>[2x]MGATGDAEQPRGPSGAERGGLELGDAGAAGQLVLTNPWNIMIKHRQVQRRGRRSQMTTSFTDPAISMDLLRAVLQPSINEEIQTVFNKYMKFFQKAALNVRDNVGEEVDAEQLIQEACRSCLEQAKLLFS;>[2x]MAQTQGTRRKVCYYYDGDVG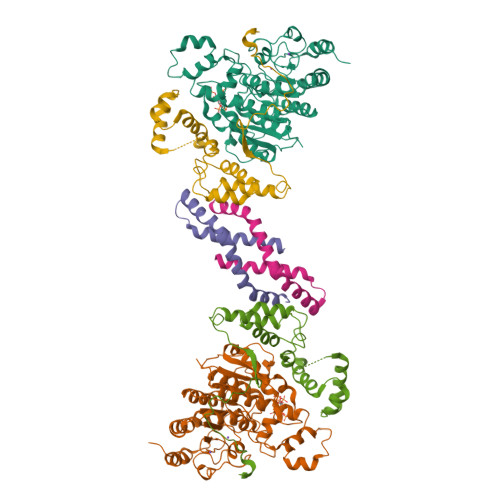NYYYGQGHPMKPHRIRMTHNLLLNYGLYRKMEIYRPHKANAEEMTKYHSDDYIKFLRSIRPDNMSEYSKQMQRFNVGEDCPVFDGLFEFCQLSTGGSVASAVKLNKQQTDIAVNWAGGLHHAKKSEASGFCYVNDIVLAILELLKYHQRVLYIDIDIHHGDGVEEAFYTTDRVMTVSFHKYGEYFPGTGDLRDIGAGKGKYYAVNYPLRDGIDDESYEAIFKPVMSKVMEMFQPSAVVLQCGSDSLSGDRLGCFNLTIKGHAKCVEFVKSFNLPMLMLGGGGYTIRNVARCWTYETAVALDTEIPNELPYNDYFEYFGPDFKLHISPSNMTNQNTNEYLEKIKQRLFENLRMLPHAPGVQMQAIPEDAIPEESGDEDEDDPDKRISICSSDKRIACEEEFSDSEEEGEGGRKNSSNFKKAKRVKTEDEKEKDPEEKKEVTEEEKTKEEKPEAKGVKEEVKLA;>GAVSIEPRINVGSRFQAEIPLMRDRALAAADPHKADLVWQPWEDLESSREKQRQVEDLLTAACSSIFPGAGTNQELALHCLHESRGDILETLNKLLLKKPLRPHNHPLATYHYTGSDQWKMAERKLFNKGIAIYKKDFFLVQKLIQTKTVAQCVEFYYTYKKQVKIGRNGTLT[2x]>[2x]STMGLLSQENTQIRDLQQENRELWISLEEHQDALELIMSKYRKQMLQLMVAKKA

Our results supported a “two-arm” architecture of the STRIPAK complex, with the PP2Aa/c-bound STRNs acting as an organizing center to hold Hippo or other MST kinases with STRIP1 as one arm and SIKE1-SLMAP as the other. Moreover, we determined the crystal structures of the second coiled-coil domain of SIKE1 alone, and in complex with an STRN3 peptide, as well as the structure of the first coiled-coil domain of SIKE1 in complex with the first coiled-coil domain of SLMAP. SIKE1 functions to bridge SLMAP through CC1 on one hand and STRN3 through CC2 on the other. In particular, we discovered SIKE1 as a key adaptor that recruits MST-bound SLMAP to PP2A-bound STRN, forming a molecular arm MST-SLMAP-SIKE1-STRN-PP2Aa/c.

To further characterize the assembly of STRN3-SIKE1 complex at the atomic level, we solved the crystal structures of SIKE1 CC2 alone (apo state) and in complex with an STRN3 peptide (residues 166–190) at 1.5 and 1.75 Å resolution, respectively. In the apo state, SIKE1 CC2 formed a symmetric homotetramer consisting of two parallel homodimers (chains A/B for one homodimer and A′/B′ for the other), namely a dimer of dimer with two dimeric units clamping each other in an antiparallel direction. As such, the N-terminal regions of SIKE1 CC2 formed a dimeric coiled coil, while the central and C-terminal regions formed a tetrameric coiled coil. Residues Q79, I80, L83, L90, W91, and L94 from each chain mediated CC2 homodimerization through hydrophobic interactions. In addition, N87 from chains A and B formed a pair of hydrogen bonds surrounding the axis of the coiled coil. Meanwhile, the four-helix bundle was stabilized by an extensive hydrophobic packing of residues L90, W91, L94, H97, L101, I104, M105, Y108, M112, L115, and M116 from each chain. Moreover, the coiled-coil assembly was further strengthened by hydrogen bonding among residues S93, L94, and Q98 from chain A, Y108 and R109 from chain B′, and Q111 from chain A′, as well as salt bridges formed between residues E102 from chain A and R109 from chain B′. As a first step, the SIKE1 CC2 homotetramer observed in the apo state would have to disassemble, producing two homodimers with an exposed binding site for STRN3. SIKE1 CC2 alone exists as a homotetramer (dimer of dimer), but forms a 2:1 heterotrimer with STRN3.(2S,3R,4S,5R)-2-METHYLPIPERIDINE-3,4,5-TRIOL | C6 H13 N O3 | 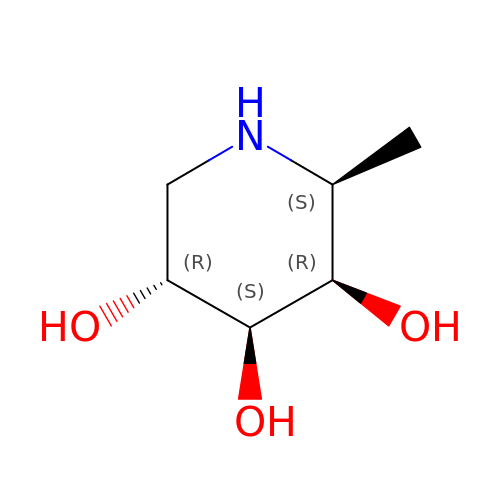VYOCYWDJTQRZLC-KCDKBNATSA-N> MKAEIKEFIDRGTYRKAPLFEGELPEGSYAQIVEIKPKQTVPKHYHEKQYELFYIISGQAKLGIEEREY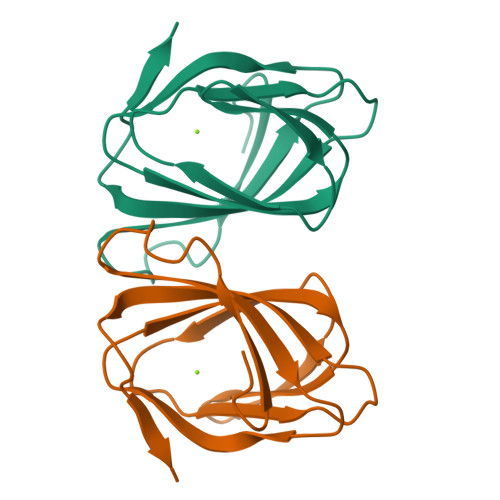DAKPGDIFLVKPKTVHWVVNKKEEPFRLFVIKLNYFGDDSVWLE>[2x]AEKPKLHYFNARGRMESTRWLLAAAGVEFEEKFIKSAEDLDKLRNDGYL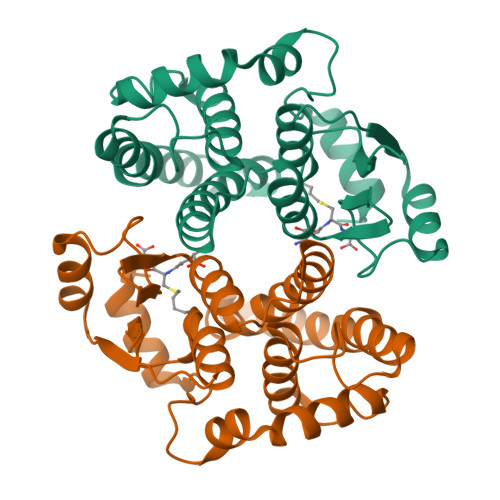MFQQVPMVEIDGMKLVQTRAALNYIASKYNLYGKDIKERALIDMYIEGIADLGEMILLLPVCPPEEKDAKLALIKEKIKNRYFPAFEKVLKSHGQDYLVGNKLSRADIHLVELLYYVEELDSSLISSFPLLKALKTRISNLPTVKKFLQPGSPRKPPMDEKSLEEARKIFRF> GDTETAIDNAIARVADTVASGPSNSTSIPALTAVETGHTSQVEPSDTMQTRHVKNYHSRSESTVENFLSRSACVYIEEYYTKDQDNVNRYMSWTINARRMVQLRRKFELFTYMRFDMEITFVITSRQLPGTSIAQDMPPLTHQIMYIPPGGPVPNSVTDFAWQTSTNPSIFWTEGNAPPRMSIPFISIGNAYSNFYDGWSHFSQNGVYGYNALNNMGKLYARHVNKDTPYQMSSTIRVYFKPKHIRVWV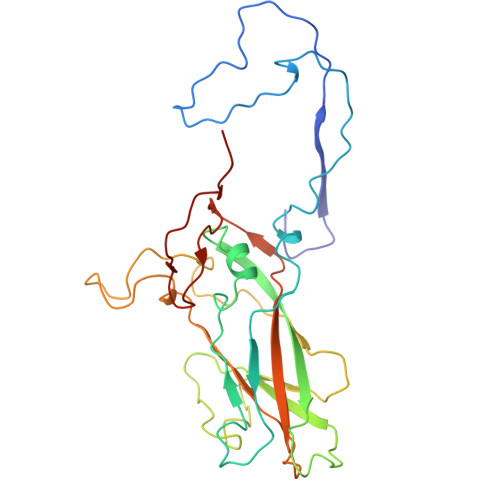PRPPRLSPYIKSSNVNFNPTNLTDERSSI>GMSWEKSGKEGSLLRWYDVMEAERYEYTVGPAGEQFFNGLKQNKIIGSKCSKCGRIFVPARSYCEHCFVKIENYVEINKDEAYVDSYTIIYNDDEGNKLAQPVYIALIRFPNIEGGLLCYAEGNVKVGAKAKILSFQWPLRVKVD[2x]

SSO2064 is the first structural representative of PF01796 (DUF35), a large prokaryotic family with a wide phylogenetic distribution. The structure reveals a novel two-domain architecture comprising an N-terminal, rubredoxin-like, zinc ribbon and a C-terminal, oligonucleotide/oligosaccharide-binding (OB) fold domain. Domain architectures, genomic context analysis and functional evidence from certain bacterial representatives of this family suggest that these proteins form a novel fatty-acid-binding component that is involved in the biosynthesis of lipids and polyketide antibiotics and that they possibly function as acyl-CoA-binding proteins. The SSO2064 gene of Sulfolobus solfataricus, a hyperthermoacidophilic crenarchaeon, encodes a protein with a molecular weight of 16.5 kDa (residues 1–144) and a calculated isoelectric point of 6.6.

The final model included residues 8–144 for chain A, residues 10–27 and 29–144 for chain B, two acetate molecules, six sulfate ions, two zinc ions and 201 water molecules in the asymmetric unit (ASU). The two molecules in th ASU are similar, with an overall Cα r.m.s.d. of 1.4 Å over 137 residues. The main differences are localized in the regions between helices H1 and H2, strands β3–β4 and strands β6–β7, which display different conformations. None of these regions are involved in crystal contacts, suggesting possible functional relevance of these conformationally flexible regions. Two N-terminal helices preceding the zinc-ribbon domain complete the structure and are involved in crystal-packing interactions. A search with PISA suggested that the likely quaternary structure of SSO2064 was either a tetramer or a dimer. However, analytical size-exclusion chromatography in combination with static light scattering strongly suggests that a monomer is likely to be the biologically relevant state of the molecule. Some of the most highly conserved residues among homologs (Pro58, Arg60, Ser82 and Thr87) line this groove, suggesting that it might serve as a binding site. We speculate that the N-terminal zinc ribbon contacts the nucleotide moiety of acyl-CoA in a manner similar to that seen in nucleic acid-binding zinc ribbons, while the hydrophobic surface of the OB fold (formed by strand β6 and loop β7–β9) could accommodate the acyl side chain. While several examples of OB-fold domains bind low-molecular-weight compounds, to our knowledge, this family appears to represent the first instance of an OB fold adapted to bind an acyl-CoA moiety.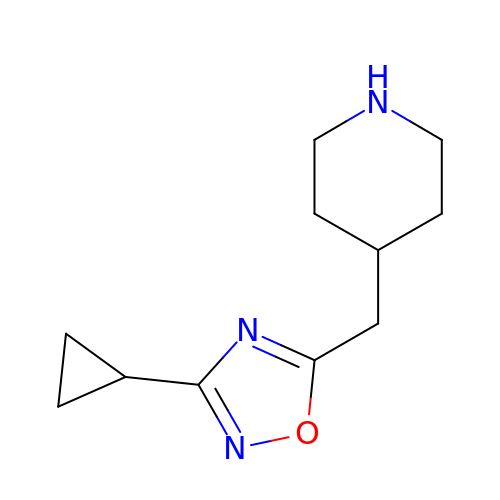4-[(3-cyclopropyl-1,2,4-oxadiazol-5-yl)methyl]piperidine | C11 H17 N3 O | UMIHXIWIKFHJRW-UHFFFAOYSA-N> SHWVX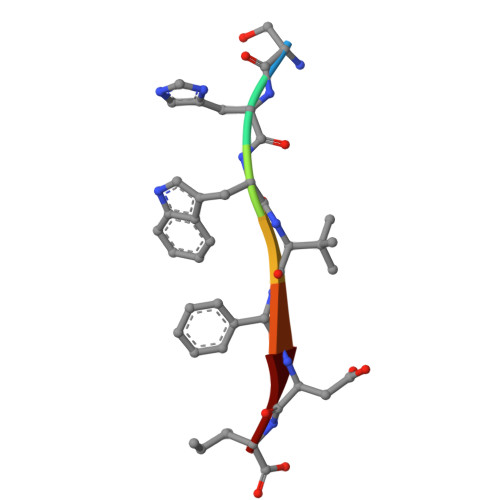DI>[2x]MNITIYDVAREANVSMATVSRVVNGNPNVKPTTRKKVLEAIERLGYRPNAVARGLASKKTTTVGVIIPDISSIFYSELARGIEDIATMYKYNIILSNSDQNMEKELHL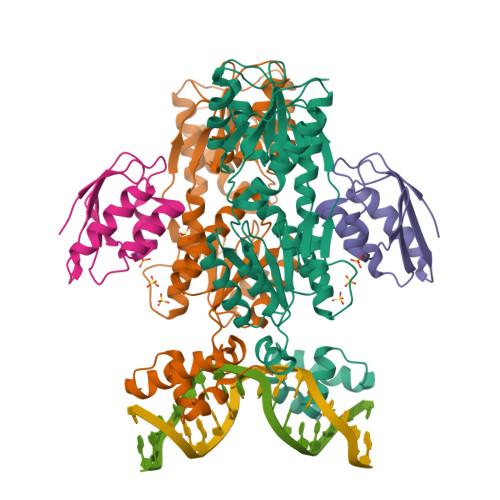LNTMLGKQVDGIVFMGGNITDEHVAEFKRSPVPIVLAASVEEQEETPSVAIDYEQAIYDAVKLLVDKGHTDIAFVSGPMAEPINRSKKLQGYKRALEEANLPFNEQFVAEGDYTYDSGLEALQHLMSLDKKPTAILSATDEMALGIIHAAQDQGLSIPEDLDIIGFDNTRLSLMVRPQLSTVVQPTYDIGAVAMRLLTKLMNKEPVEEHIVELPHRIELRKSTKAHHHHHH;>[2x]AQKTFKVTADSGIHARPATVLVQTASKYDADVNLEYNGKTVNLKSIMGVMSLGIAKGAEITISASGADENDALNALEETMKSEGLGE>MTSGDKETPKREDFASALRFLMGGCAREPEMTAMAPLNLPKKWARILRMSSTPKIPIVDYLEAAESGNLDDFKRLFMADNSRIALKDAKGRTAAHQAAARNRVNILRYIRDQNGDFNAKDNAGNTPLHIAVESDAYDALD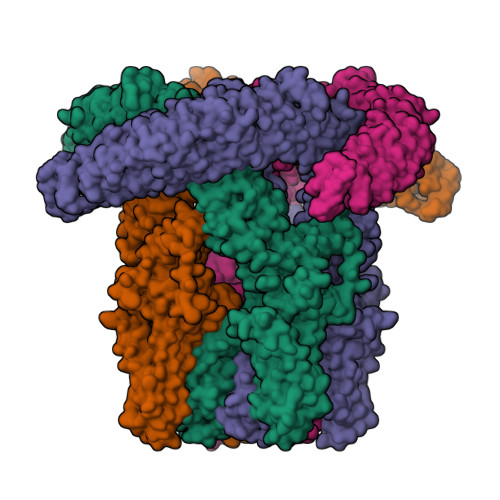YLLSIPVDTGVLNEKKQAPVHLATELNKVKSLRVMGQYRNVIDIQQGGEHGRTALHLAAIYDHEECARILITEFDACPRKPCNNGYYPIHEAAKNASSKTMEVFFQWGEQRGCTREEMISFYDSEGNVPLHSAVHGGDIKAVELCLKSGAKISTQQHDLSTPVHLACAQGAIDIVKLMFEMQPMEKRLCLSCTDVQKMTPLHCASMFDHPDIVSYLVAEGADINALDKEHRSPLLLAASRSGWKTVHLLIRLGACISVKDAAARNVLHFVIMNGGRLTDFAEQVANCQTQAQLKLLLNEKDSMGCSPLHYASRDGHIRSLENLIRLGACINLKNNNNESPLHFAARYGRYNTVRQLLDSEKGSFIINESDGAGMTPLHISSQQGHTRVVQLLLNRGALLHRDHTGRNPLQLAAMSGYTETIELLHSVHSHLLDQVDKDGNTALHLATMENKPHAISVLMSMGCKLVYNVLDMSAIDYAIYYKYPEAALAMVTHEERANEVMALRSDKHPCVTLALIASMPKVFEAVQDKCITKANCKKDSKSFYIKYSFAFLQCPFMFAKIDEKTGESITTASPIPLPALNTMVTHGRVELLAHPLSQKYLQMKWNSYGKYFHLANLLIYSIFLVFVTIYSSLMMNNIELKAGDNKTMSQYCNMGWEQLTMNLSQNPSVASQIRLDSCEERINRTTAILFCAVVIVVYILLNSMRELIQIYQQKLHYILETVNLISWVLYISALVMVTPAFQPDGGINTIHYSAASIAVFLSWFRLLLFLQRFDQVGIYVVMFLEILQTLIKVLMVFSILIIAFGLAFYILLSKIIDPQPNHLSFSNIPMSLLRTFSMMLGELDFVGTYVNTYYRDQLKVPMTSFLILSVFMILMPILLMNLLIGLAVGDIESVRRNAQLKRLAMQVVLHTELERKLPHVWLQRVDKMELIEYPNETKCKLGFCDFILRKWFSNPFTEDSSMDVISFDNNDDYINAELERQRRKLRDISRMLEQQHHLVRLIVQKMEIKTEADDVDEGISPNELRSVVGLRSAGGNRWNSPRVRNKLRAALSFNKSM[4x]>[2x]GSHETNTIFKLE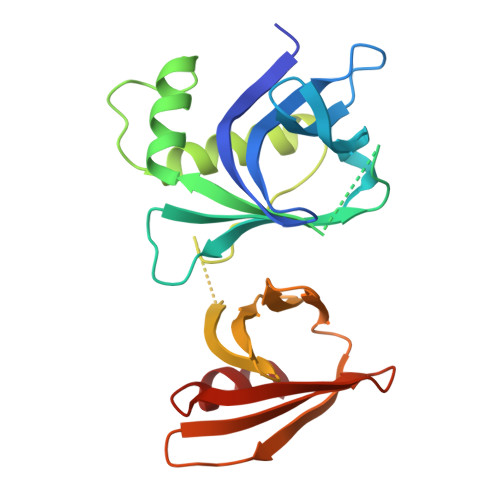GVSVLSPLRKKLDLVFYLSNVDGSPVITLLKGNDRELSIYQLNKNIKMASFLPVPEKPNLIYLFMTYTSCEDNKFSEPVVMTLNKENTLNQFKNLGLLDSNVTDFEKCVEYIRKQAILTGFKISNPFVNSTLVDTDAEKINSFHLQCHRGTKEGTLYFLPDHIIFGFKKPILLFDASDIESITYSSITRLTFNASLVTKDGEKYEFSMIDQTEYAKIDDYVKR>[2x]MYKGISAANYAASNIE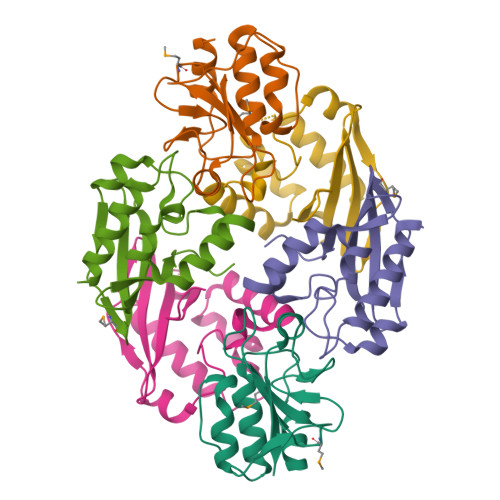PNSVGRCAEYVRKAIEWGGISLQRTRSAKDYGPSLLAAGFHEAIGSPMKGDVIVIQPAPGHPHGHMAIYDGSHWISDFKQLHGFYPGPAYRSAKPAYKTYRYH;>MGSSHHHHHHENLYFQGHMGSAQAAVSQNSPEAAAISFYTWFIQHDSDQTYPLSEPDIERYVATDTVGRLRNDYAHAGPPNGVDYFLKVQDYDSRDWLAHIQVQRALMLGDVAVVPVSFGSQDPVHVLVFLKRVDATWKIIKIDDTWEYR[4x]> MAVKRPVRVLVNMDGVLADFESGLLQGFRRRFPEEPHVPLEQRRGFLANEQYGALRPDLAEKVASVYESPGFFLNLEPIPGALDALREMNDMKDTEVFICTTPLL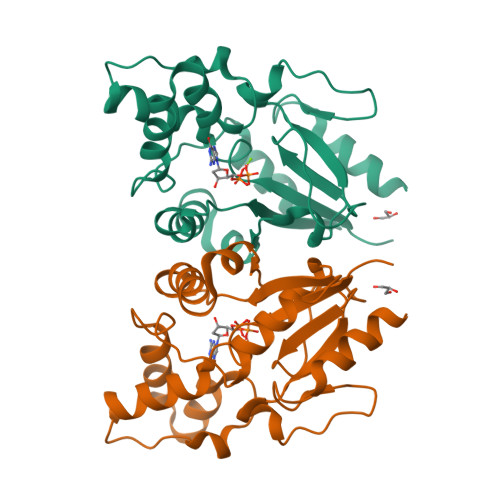KYDHCVGEKYRWVEQNLGPEFVERIILTRDKTVVMGDLLIDDKDNIQGLEETPSWEHILFTCCHNQHLALPPTRRRLLSWSDNWRGIIESKRASL> KAQ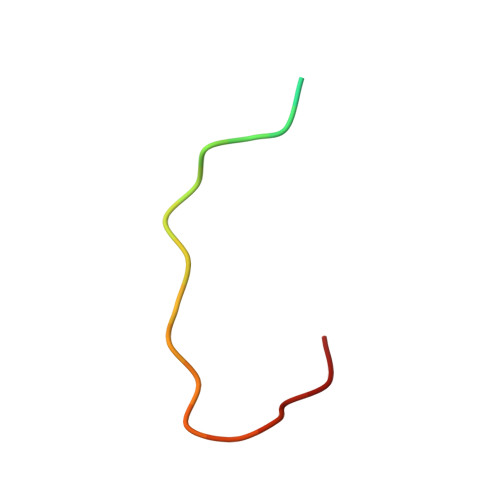KKNRNKLRRQHDYDTFVDL>MSSRSDPGQPMASATDPSGRLALDLTECDREPIHIPGAIQPHGYLFVVSETDLRIASVSANVEDLLRQPPASLLNVPIAHYLTAASAARLTHALHGGDPAAINPIRLDVVTPDGERAFNGILHRHDSIVILELEPRDESRYTNEFFRSVRVAIRRLQTAADLPTACWIAASEVRRITGFDRIKVYQFAADWSGQVIAEDRDSGIPSLLDFHFPSSDIPAQSRALYTINPVRIIPDIGYRPSPLVPDINPRLGGPIDLSFSVLRSVSPTHLEYMVNMGMHAAMSISIVRDNRLWGMISCHNLTPRFVSYEVRQA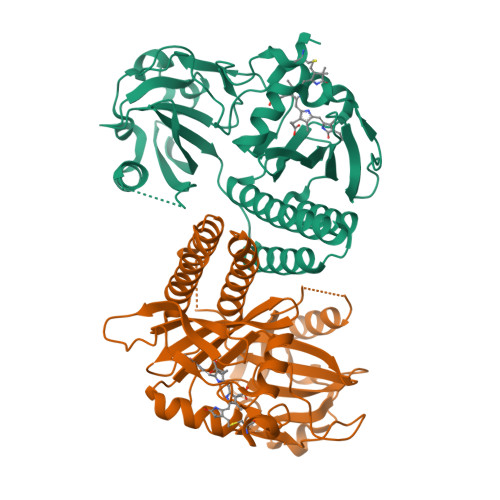CELIAQVLTWQIGVLEEAEIVRHS[2x]DAHP Oxime | C7 H14 N O10 P | 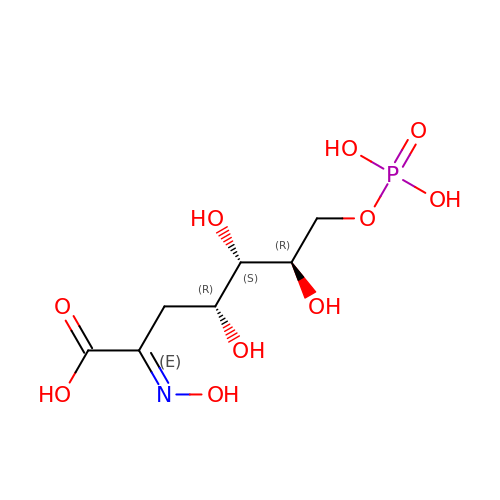KFGHSGKOOHKNEU-WVMCLEPLSA-N>MSEFNITETYLRFLEEDTEMTMPIAAIEALVTLLRIKTPETAAEMINTIKSSTEELIKSIPNSVSLRAGCDIFMRFVLRNLHLYGDWENCKQHLIENGQLFVSRAKKSRNKIAEIGVDFIADDDIILVHGYSRAVFSLLNHAANKFIRFRCVVTESRPSKQGNQLYTLLEQKGIPVTLIVDSAVGAVIDKVDKVFVGAEGVAESGGIINLVGTYSVGVLAHNARKPFYVVTESHKFVRMFPLSSDDLPMAGPPLDFTRRTDDLEDALRGPTIDYTAQEYITALITDLGVLTPSAVSEELIKMWYD[2x];>[2x]MSSQAFTSVHPNAATSDVNVTIDTFVAKLKRRQVQGSYAIALETLQLLMRFISAARWNHVNDLIEQIRDLGNSLEKAHPTAFSCGNVIRRILAVLRDEVEEDTMSTTVTSTSVAEPLISSMFNLLQKPEQPHQNRKNSSGSSSMKTKTDYRQVAIQGIKDLIDEIKNIDEGIQQIAIDLIHDHEILLTPTPDSKTVLKFLITARERSNRTFTVLVTEGFPNNTKNAHEFAKKLAQHNIETLVVPDSAVFALMSRVGKVIIGTKAVFVNGGTISSNSGVSSVCECAREFRTPVFAVAGLYKLSPLYPFDVEKFVEFGGSQRILPRMDPRKRLDTVNQITDYVPPENIDIYITNVGGFNPSFIYRIAWDNYKQIDVHLDKNKA;>MSIQAFVFCGKGSNLAPFTQPDFPFQTQNKDSTAATSGDKLNELVNSALDSTVINEFMQHSTRLPKALLPIGNRPMIEYVLDWCDQADFKEISVVAPVDEIELIESGLTSFLSLRKQQFELIYKALSNSNHSHHLQDPKKINFIPSKANSTGESLQKELLPRINGDFVILPCDFVTDIPPQVLVDQFRNRDDNNLAMTIYYKNSLDSSIDKKQQQKQKQQQFFTVYSENEDSERQPILLDVYSQRDVTKTKYLQIRSHLLWNYPNLTVSTKLLNSFIYFCSFELCQLLKLGPQSMSRQASFKDPFTGNQQQQNPPTTDDDEDRNHDDDDDYKPSATSIQPTYFKKKNDLILDPINCNKSLSKVFRDLSRRSWQHSKPREPIGIFILPNETLFIRANNLNAYMDANRFVLKIKSQTMFTKNIQIQSAAIGADAIVDPKCQISAHSNVKMSVLGTQANIGSRCRVAGSLLFPGVHLGDEVILENCIIGPMAKIGSKCKLSNCYIEGHYVVEPKNNFKGETLANVYLDEDEEDELIYDDSVIAGESEIAEETDSDDRSDEDSDDSEYTDEYEYEDDGLFER[2x];>[2x]MSESEAKSRSATPPSKAKQATPTTTAAANGEKKLTNKELKELKKQEKAAKRAAMKQANGISIEQQQQQAQMKKEKKQLQREQQQKREQKQKNANKKKQNERNVKKSTLFGHLETTEERRATILALTSAVSSPKTSRITAAGLMVPVVASALSGSNVLTASSLMPVGPNASSTVSASAPASTTTTLPASSAALSAGTSSASTNTPTAIQQEIASSNASDVAKTLASISLEAGEFNVIPGISSVIPTVLEQSFDNSSLISSVKELLLNKDLIHPSILLLTSHLAHYKIVGSIPRCIAMLEVFQIVIKDYQTPKGTTLSRNLTSYLSHQIDLLKKARPLSVTMGNAIRWLKQEISLIDPSTPDKAAKKDLCEKIGQFAKEKIELADQLIIDNASTQIEESTTIVTYGSSKVLTELLLHNAISLKKNIKVIVVDSRPLFEGRKMAETLRNAGVNVMYALITSLDTIFNMDVDYVFLGAHSILSNGFLYSRAGTAMLAMSAKRRNIPVLVCCESLKFSQRVQLDSVTFNELADPNDLVNIDYENPVERRGNKGALLNQFIKERKFEKKKLAMENKPKGNKIGGKKGSEGESKDASNEEDSNSKNILDGWQELPSLNIVNILYDLTPPEYIKKVITEFGALPPSSVPVILREYKGSA;>MAGKKGQKKSGLGNHGKNSDMDVEDRLQAVVLTDSYETRFMPLTAVKPRCLLPLANVPLIEYTLEFLAKAGVHEVFLICSSHANQINDYIENSKWNLPWSPFKITTIMSPEARCTGDVMRDLDNRGIITGDFILVSGDVLTNIDFSKMLEFHKKMHLQDKDHISTMCLSKASTYPKTRTIEPAAFVLDKSTSRCIYYQDLPLPSSREKTSIQIDPELLDNVDEFVIRNDLIDCRIDICTSHVPLIFQENFDYQSLRTDFVKGVISSDILGKHIYAYLTDEYAVRVESWQTYDTISQDFLGRWCYPLVLDSNIQDDQTYSYESRHIYKEKDVVLAQSCKIGKCTAIGSGTKIGEGTKIENSVIGRNCQIGENIRIKNSFIWDDCIIGNNSIIDHSLIASNATLGSNVRLNDGCIIGFNVKIDDNMDLDRNTKISASPLKNAGSRMYDNESNEQFDQDLDDQTLAVSIVGDKGVGYIYESEVSDDEDSSTEACKEINTLSNQLDELYLSDDSISSATKKTKKRRTMSVNSIYTDREEIDSEFEDEDFEKEGIATVERAMENNHDLDTALLELNTLRMSMNVTYHEVRIATITALLRRVYHFIATQTLGPKDAVVKVFNQWGLLFKRQAFDEEEYIDLMNIIMEKIVEQSFDKPDLILFSALVSLYDNDIIEEDVIYKWWDNVSTDPRYDEVKKLTVKWVEWLQNADEESSSEEE[2x];>[2x]MSTSHCRFYENKYPEIDDIVMVNVQQIAEMGAYVKLLEYDNIEGMILLSELSRRRIRSIQKLIRVGKNDVAVVLRVDKEKGYIDLSKRRVSSEDIIKCEEKYQKSKTVHSILRYCAEKFQIPLEELYKTIAWPLSRKFGHAYEAFKLSIIDETVWEGIEPPSKDVLDELKNYISKRLTPQAVKIRADVEVSCFSYEGIDAIKDALKSAEDMSTEQMQVKVKLVAAPLYVLTTQALDKQKGIEQLESAIEKITEVITKYGGVCNITMPPKAVTATEDAELQALLESKELDNRSDSEDDEDESDDE;>MSDLQDQEPSIIINGNLEPVGEPDIVEETEVVAQETQETQDADKPKKKVAFTGLEEDGETEEEKRKREFEEGGGLPEQPLNPDFSKLNPLSAEIINRQATINIGTIGHVAHGKSTVVRAISGVQTVRFKDELERNITIKLGYANAKIYKCQEPTCPEPDCYRSFKSDKEISPKCQRPGCPGRYKLVRHVSFVDCPGHDILMSTMLSGAAVMDAALLLIAGNESCPQPQTSEHLAAIEIMKLKHVIILQNKVDLMREESALEHQKSILKFIRGTIADGAPIVPISAQLKYNIDAVNEFIVKTIPVPPRDFMISPRLIVIRSFDVNKPGAEIEDLKGGVAGGSILNGVFKLGDEIEIRPGIVTKDDKGKIQCKPIFSNIVSLFAEQNDLKFAVPGGLIGVGTKVDPTLCRADRLVGQVVGAKGHLPNIYTDIEINYFLLRRLLGVKTDGQKQAKVRKLEPNEVLMVNIGSTATGARVVAVKADMARLQLTSPACTEINEKIALSRRIEKHWRLIGWATIKKGTTLEPIA[2x];>MSSDLAAELGFDPALKKKKKTKKVIPDDFDAAVNGKENGSGDDLFAGLKKKKKKSKSVSADAEAEKEPTDDIAEALGELSLKKKKKKTKDSSVDAFEKELAKAGLDNVDAESKEGTPSANSSIQQEVGLPYSELLSRFFNILRTNNPELAGDRSGPKFRIPPPVCLRDGKKTIFSNIQDIAEKLHRSPEHLIQYLFAELGTSGSVDGQKRLVIKGKFQSKQMENVLRRYILEYVTCKTCKSINTELKREQSNRLFFMVCKSCGSTRSVSSIKTGFQATVGKRRRM[2x]

For multiple rounds of initiation to occur, the GDP on eIF2 has to be exchanged for GTP. This reaction is catalysed by a guanine nucleotide exchange factor (GEF) eIF2B. Here we have determined a cryoEM structure of eIF2B in complex with the GDP-bound form of eIF2 phosphorylated at Ser51 on the α subunit, which sheds light on the molecular interactions between the two molecules and provides a basis for understanding the regulation of translation by eIF2α phosphorylation. The structure consists of two eIF2 molecules bound to opposite sides of the eIF2B hetero-decamer.

To improve resolution in this region, we combined particles from both datasets and carried out 3D EM data classification applying a twofold C2 symmetry and using masks around eIF2 molecules in the complex. This classification resulted in map 2 with slightly lower overall resolution 4.3 Å, however, the local resolution for eIF2γ and eIF2α-D3 was better compared to map 1. In a low-resolution filtered map 2 contoured at lower threshold, we could see weak densities around eIF2γ, which cannot be attributed to this subunit (blue and red masks). Each eIF2 molecule has two spatially separated interactions with the eIF2B hetero-decamer—one through eIF2α-D1 inserted in the pocket between eIF2B α and δ subunits and another contact of eIF2γ with the catalytic eIF2B subunits. Another contact is formed by eIF2γ and eIF2β interacting with the catalytic eIF2B subunits γ and ε. Although eIF2α-D1 containing the phosphorylated Ser51 is relatively constrained through its interaction with eIF2B, the domains eIF2 γ and β in the proximity of the catalytic portion of eIF2B have relatively high conformational heterogeneity presumably arising from high mobility and do not adopt the same conformation in two eIF2 molecules bound on either side of eIF2B.> MGSSHHH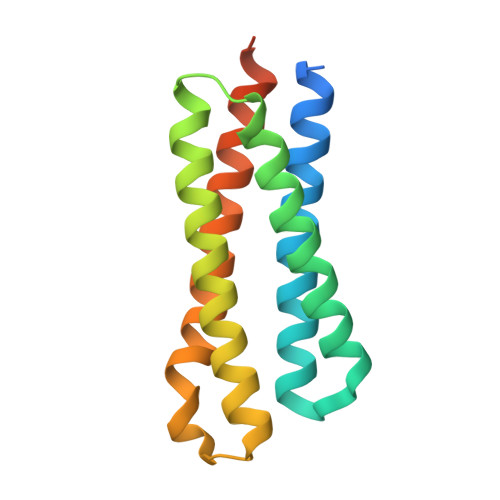HHHSQGSMLNNMLITNEIKQHVDSSLDNFNQYILNGTPSKKESYNNEVILAKQKIGNLKKNSDDVNQYILRDLDNTLDSYIESSKNTISAYENKEGYVFYYDDFVAAKNIASYCDAYASTLMQNFLEANSIAYKELNRNSS> INSSSVSTALKVAGAILKFVNPPAGTVLTVLSAVLPILWPTNTPTPERVWNDFMTNTGNLIDQTVTAYVRTDANAKMTVVKDYLDQYTTKFNTWKREPNNQSYRTAVITQFNLTSAKLRETAVYFSNLVGYELLLLPIYAQVANFNLLLIRDGLINAQEWSLAQSAGDQLYNTMVQYTKEYIAHSITWYNKGLDVLRNKSNGQWITFNDYKREMTIQVLDILALFASYDPRRYPADKIDNTKLSKTEFTREIYTALVESPSSKSIAALEAALTRDVHLFTWLKRVDF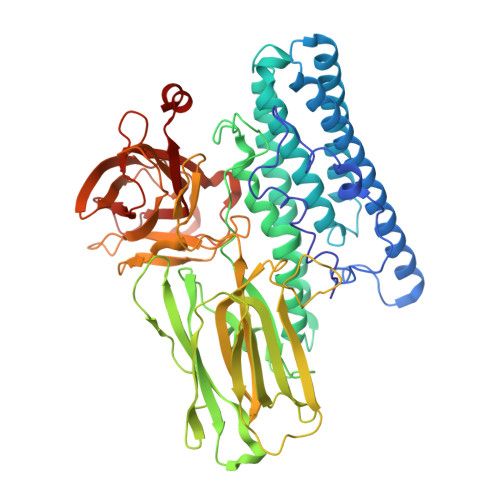WTNTIYQDLRFLSANKIGFSYTNSSAMQESGIYGSSGFGSNLTHQIQLNSNVYKTSITDTSSPSNRVTKMDFYKIDGTLASYNSNITPTPEGLRTTFFGFSTNENTPNQPTVNDYTHILSYIKTDVIDYNSNRVSFAWTHKIVDPNNQIYTDAITQVPAVKSNFLNATAKVIKGPGHTGGDLVALTSNGTLSGRMEIQCKTSIFNDPTRSYGLRIRYAANSPIVLNVSYVLQGVSRGTTISTESTFSRPNNIIPTDLKYEEFRYKDPFDAIVPMRLSSNQLITIAIQPLNMTSNNQVIIDRIEIIPITQSVLDET6-{[(1R,2S)-2-aminocyclohexyl]amino}-7-fluoro-4-(1-methyl-1H-pyrazol-4-yl)-1,2-dihydro-3H-pyrrolo[3,4-c]pyridin-3-one 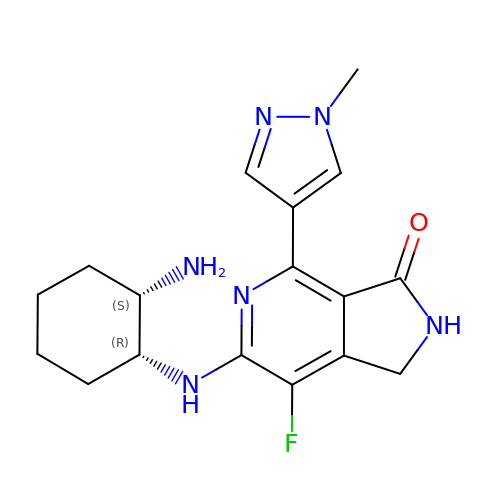| C17 H21 F N6 O | MJHOMTRKVMKCNE-NWDGAFQWSA-N>KTPPVVFHWFPFIGSTISYGIDPYKFFFDCRAKYGDIFTFILLGKKTTVYLGTKGNDFILNGKLRDVCAEEVYSPLTTPVFGRHVVYDCPNAKLMEQKKFVKYGLTSDALRSYVPLITDEVESFVKNSPAFQGHKGVFDVCKTIAEITIYTASRSLQGKEVRSKFDSTFAELYHNLDMGFAPINFMLPWAPLPHNRKRDAAQRKLTETYMEIIKARRQAGSKKDSEDMVWNLMSCVYKNGTPVPDEEIAHMMIALLMAGQHSSSSTASWIVLRLATRPDIMEELYQEQIRVLGSDLPPLTYDNLQKLDLHAKVIKETLRLHAPIHSIIRAVKNPMAVDGTSYVIPTSHNVLSSPGVTARSEEHFPNPLEWNPHRWDENIAASAEDDEKVDYGYGLVSKGTNSPYLPFGAGRHRCIGEQFAYLQ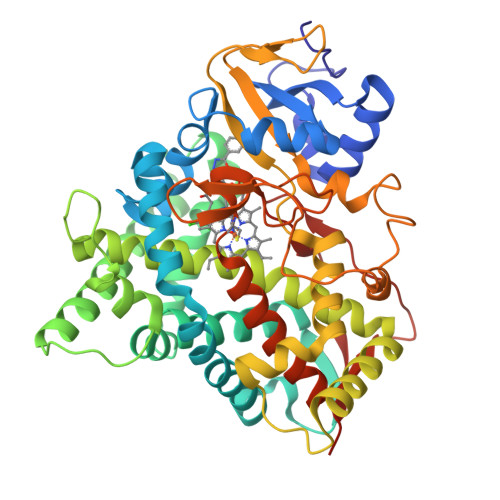LGTITAVLVRLFRFRNLPGVDGIPDTDYSSLFSKPLGRSFVEFEKRH[2x]> TTRDRVPTYQYNMNFEKLGKCIIINNKNFDKVTGMGVRNGTDKDAEALFKCFRSLGFDVIVYNDCSCAKMQDLLKKASEEDHTNAACFACILLSHGEENVIYGKDGVTPIKDLTAHFRGDRSKTLLEKPKLFFIQACRGTELDDGIQADSGPINDTDANPRYKAPVEADFLFAYSTVPGYYSWRSPGRGSWFVQALCSILEEHGKDLEIM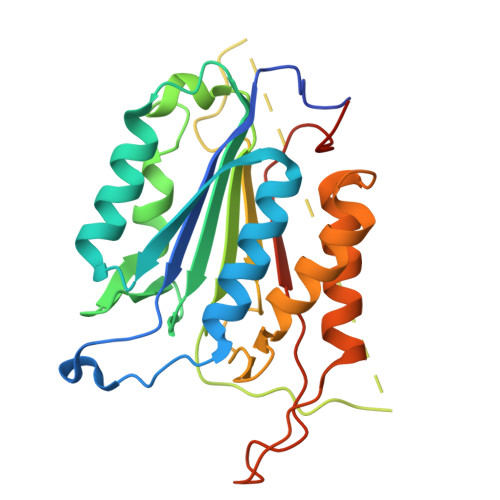QILTRVNDRVARHFESQSDDPHFHEKKQIPCVVSMLTKELYFSQHHHHHH>MKVISFLNPKGGSGKTTAVINIATALSRSGYNIAVVDTDPQMSLTNWSKAGKAAFDVFTAASEKDVYGIRKDLADYDFAIVDGAGSLSVITSAAVMVSDLVIIPVTPSPLDFSAAGSVVTVLEAQAYSRKVE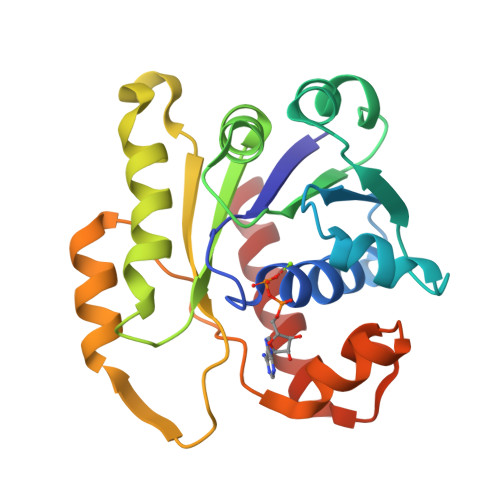ARFLITRKIEMATMLNVLKESIKDTGVKAFRTAITQRQVYVKSILDGDSVFESSDGAAKGEIEILTKEIVRIFE[2x]>GSAKNSSNRMYMEKSQTELGDLSDTLLSKVDDLQDVIEIMRKDVAERRSQPAKKKLETVSKDLENAQADVLKLQEFIDTEKPHWKKTWEAELDKVCEEQQFLTLQEELILDLKEDLG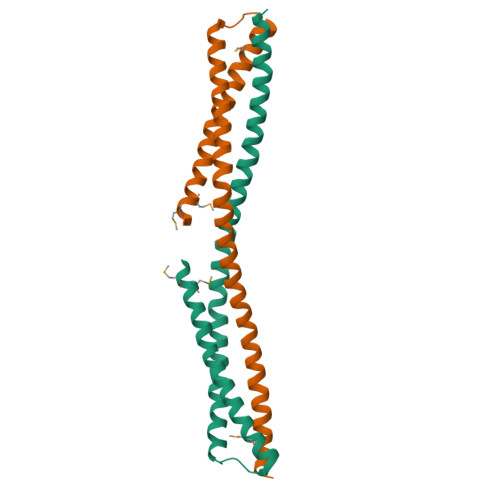KALETFDLIKLCCEEQEKNPSRSK[2x]> MSRSKRDNNFYSVEIGDSTFTVLKRYQNLKPIGSGAQGIVVAAYDAILERNVAIKKLSRPFQNQTHAKRAYRELVLMKVVNHKNIIGLLNVFTPQKSLEEFQ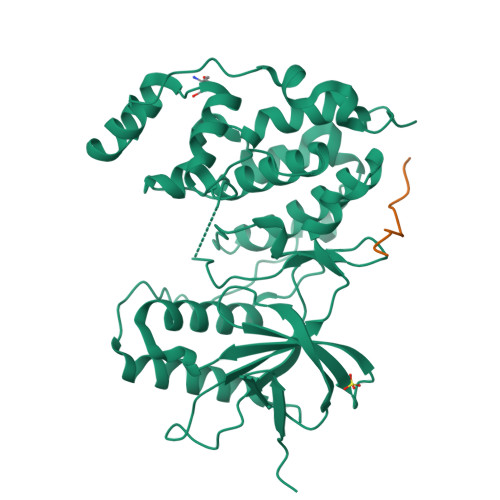DVYIVMELMDANLSQVIQMELDHERMSYLLYQMLVGIKHLHSAGIIHRDLKPSNIVVKSDATLKILDFGLARTAGTSFMMTPYVVTRYYRAPEVILGMGYKENVDIWSVGVIMGEMIKGGVLFPGTDHIDQWNKVIEQLGTPSPEFMKKLQPTVRTYVENRPKYAGYSFEKLFPDVLFPADSEHNKLKASQARDLLSKMLVIDASKRISVDEALQHPYINVWYDPSEAEAPPPKIPDKQLDEREHTIEEWKELIYKEVMDLEHHHHHH;> RPKRPTTLNLF>[5x]MTTRKESELEGVTLLGNQGTNYLFEYAPDVLESFPNKHVNRDYFVKFNCPEFTSLAPK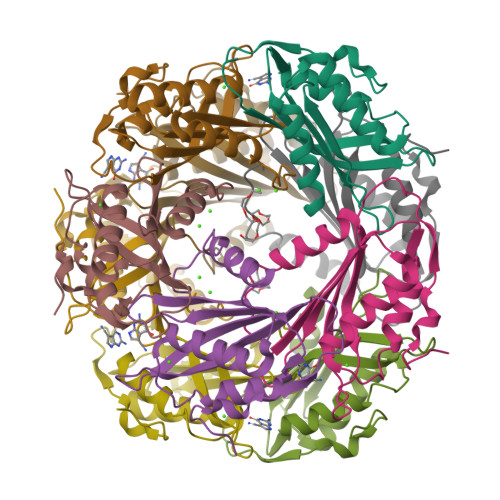TGQPDFATIYISYIPDEKMVESKSLKLYLFSFRNHGDFHEDCMNIIMNDLIELMDPRYIEVWGKFTPRGGISIDPYTNYGKPGTKYEKMAEYRMMNHDLYPETIDNR>[2x]GGADQKGPVFLKEPTNRIDFSNSTGAEIECKASGNPMPEIIWIRSDGTAVGDVPGLRQISSDGKLVFPPFRAEDYRQEVHAQVYACLARNQFGSIISRDVHVRAVVAQYYEADVNKEHVIRGNSAVIKCLIPSF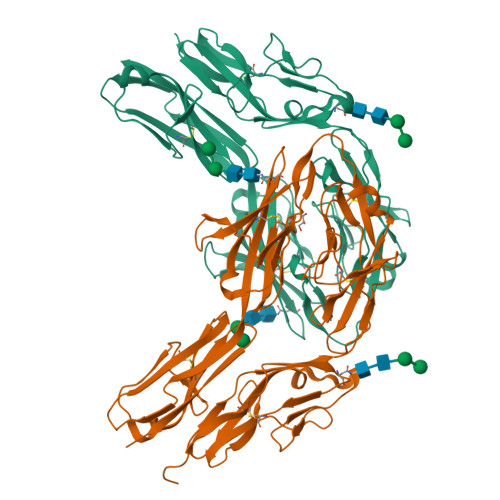VADFVEVVSWHTDEEENYFPGAEYDGKYLVLPSGELHIREVGPEDGYKSYQCRTKHRLTGETRLSATKGRLVITEPVGSVRPKVNPQDKHQFIDVELASSYSLLCMAQSYPTPSFRWYKFIEGTTRKQAVVLNDRVKQVSGTLIIKDAVVEDSGKYLCVVNNSVGGESVETVLTVTAPLSAKIDPPTQTVDFGRPAVFTCQYTGNPIKTVSWMKDGKAIGHSEPVLRIESVKKEDKGMYQCFVRNDQESAEASAELKLGG> MILDADYITEDGKPIIRIFKKENGEFKVEYDRNFRPYIYALLKDDSQIDEVRKITAERHGKIVRIIDAEKVRKKFLGRPIEVWRLYFEHPQDVPAIRDKIREHSAVIDIFEYDIPFAKRYLIDKGLIPMEGDEELKLLAFDIETLYHEGEEFAKGPIIMISYADEEEAKVITWKKIDLPYVEVVSSEREMIKRFLKVIREKDPDVIITYNGDSFDLPYLVKRAEKLGIKLPLGRDGSEPKMQRLGDMTAVEIKGRIHFDLYHVIRRTINLPTYTLEAVYEAIFGKPKEKVYAHEIAEAWETGKGLERVAKYSMEDAKVTYELGREFFPMEAQLSRLVGQPLWDVSRSSTGNLVEWYLLRKAYERNELAPNKPDEREYERRLRESYAGGYVKEPEKGLWEGLVSLDFRSLYPSIIITHNVSPDTLNREGCREYDVAPEVGHKFCKDFPGFIPSLLKRLLDERQEIKRKMKASKDPIEKKMLDYRQRAIKILANSYYGYYGYAKARWYCKECAESVTAWGREYIEFVRKELEEKFGFKVLYIDTDGLYATIPGAKPEEIKKKALEFVDYINAKLPGLLELEYEGFYVRGFFVTKKKYALIDEEGKIITRGLEIVRRDWSEIAKETQAKVLEAILKHGNVEEAVKIVKEVTEKLSKYEIPPEKLVIYEQITRPLHEYKAIGPHVAVAKRLAARGVKVRPGMV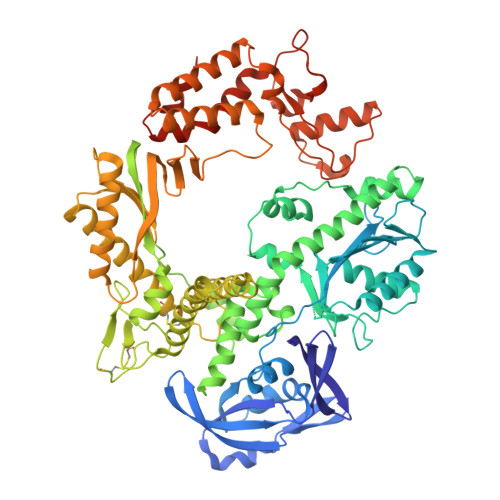IGYIVLRGDGPISKRAILAEEFDLRKHKYDAEYYIENQVLPAVLRILEAFGYRKEDLRWQKTKQTGLTAWLNIKKK>STMALLSQENTQIRDLQQENRELWISLEEHQDALELIMSKYRKQMLQLMVAKKA[2x];> PQNSQLTWK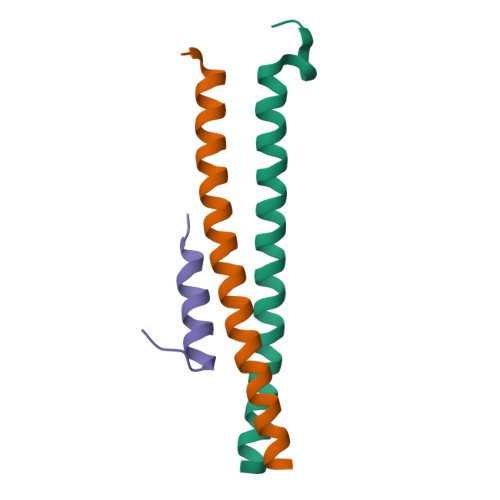QGRQLLRQYLQEVGYTD4-(2,3-dihydroindol-1-yl)-4-oxidanylidene-butanoic acid | C12 H13 N O3 | 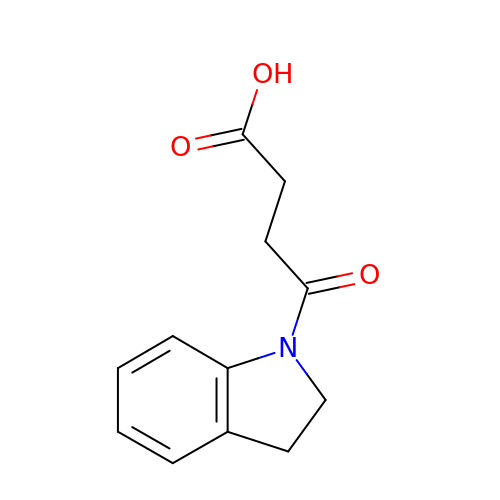SWNRXQYQTQVWKA-UHFFFAOYSA-N> MDSIDEQIAIKRKELQ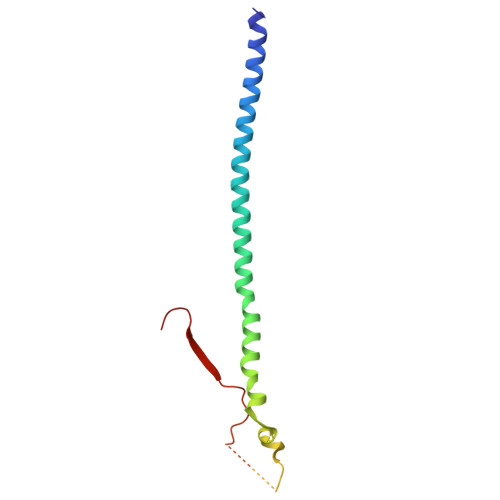SLQKITSLTDGLKIQLTELNEQIKEMGMNADSVAQLMNNWDSIINNISQASLGLLQYAEGDYEIGPWKDSKKKESEQSNETGLEAQENDKNDEDNDEDEDLVPLPETMVRIRVDGNE> MAWSHPQFEKSRPFKLPKSYAALIADWPVVVLGMCTMFIVVCALVGVLVPELPDFSDPLLGFEPRGTAIGQRLVTWNNMVKNTGYKATLANYPFKYADEQAKSHRDDRWSDDHYEREKREVDWNFHKDSFFCDVPSDRYSRVVFTSSGGETLWNLPAIKSMCNVDNSRIRSHPQFGDLCQRTTAASCCPSWTLGNYIAILNNRSSCQKIVERDVSHTLKLLRTCAKHYQNGTLGPDCWDMAARRKDQLKCTNVPRKCTKYNAVYQILHYLVDKDFMTPKTADYATPALKYSMLFSPTEKGESMMNIYLDNFENWNSSDGVTTITGIEFGIKHSLFQDYLLMDTVYPAIAIVIVLLVMCVYTKSMFITLMT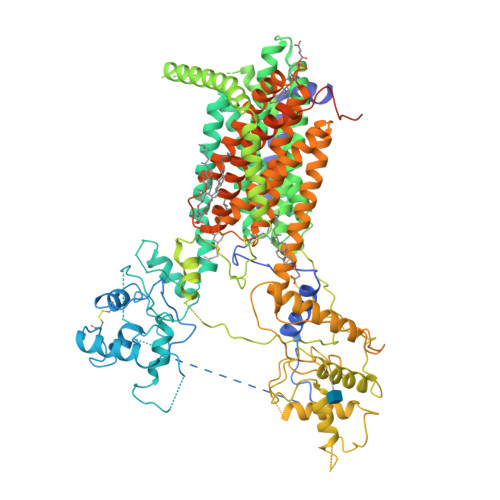MFAIISSLIVSYFLYRVVFHFEFFPFMNLTALIILVGIGADDAFVLCDVWNYTKFDKPHAETSETVSITLQHAALSMFVTSFTTAAAFYANYVSNITAIRCFGVYAGTAILVNYVLMVTWLPAVVVLHERYLLNIFTCFKKPQQQIYDNKSCWTVACQKCHKVLFAISEASRIFFEKVLPCIVIKFRYLWLFWFLALTVGGAYIVCINPKMKLPSLELSEFQVFRSSHPFERYDAEYKKLFMFERVHHGEELHMPITVIWGVSPEDNGNPLNPKSKGKLTLDSSFNIASPASQAWILHFCQKLRNQTFFYQTDEQDFTSCFIETFKQWMENQDCDEPALYPCCSHWSFPYKQEIFELCIKRAIMELERSTGYHLDSKTPGPRFDINDTIRAVVLEFQSTYLFTLAYEKMHQFYKEVDSWISSELSSAPEGLSNGWFVSNLEFYDLQDSLSDGTLIAMGLSVAVAFSVMLLTTWNIIISLYAIISIAGTIFVTVGSLVLLGWELNVLESVTISVAVGLSVDFAVHYGVAYRLAPDPDREGKVIFSLSRVGSAMAMAALTTFVAGAMMMPSTVLAYTQLGTFMMLIMCISWAFATFFFQCMCRCLGPQGTCGQIPLPKKLQCSAFSHALSTSPSDKGQSKTHTINAYHLDPRGPKSELEHEFYELEPLASHSCTAPEKTTYEETHICSEFFNSQAKNLGMPVHAAYNSELSKSTESDAGSDYKDDDDK> MLHAFTNQYQLSKTLRFGATLKEDEKKCKSHEELKGFVDISYENMKSSATIAESLNENELVKKCERCYSEIVKFHNAWEKIYYRTDQIAVYKDFYRQLSRKARFDAGKQNSQLITLASLCGMYQGAKLSRYITNYWKDNITRQKSFLKDFSQQLHQYTRALEKSDKAHTKPNLINFNKTFMVLANLVNEIVIPLSNGAISFPNISKLEDGEESHLIEFALNDYSQLSELIGELKDAIATNGGYTPFAKVTLNHYTAEQKPHVFKNDIDAKIRELKLIGLVETLKGKSSEQIEEYFSNLDKFSTYNDRNQSVIVRTQCFKYKPIPFLVKHQLAKYISEPNGWDEDAVAKVLDAVGAIRSPAHDYANNQEGFDLNHYPIKVAFDYAWEQLANSLYTTVTFPQEMCEKYLNSIYGCEVSKEPVFKFYADLLYIRKNLAVLEHKNNLPSNQEEFICKINNTFENIVLPYKISQFETYKKDILAWINDGHDHKKYTDAKQQLGFIRGGLKGRIKAEEVSQKDKYGKIKSYYENPYTKLTNEFKQISSTYGKTFAELRDKFKEKNEITKITHFGIIIEDKNRDRYLLASE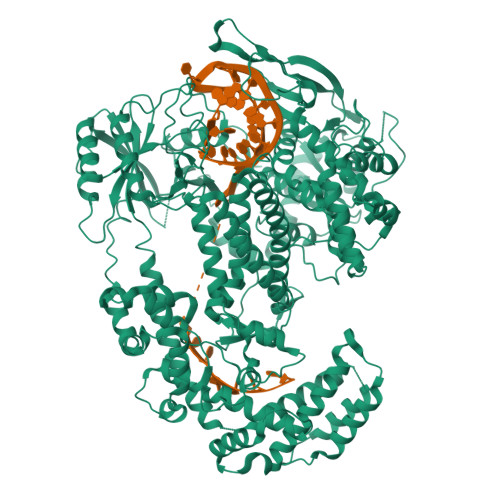LKHEQINHVSTILNKLDKSSEFITYQVKSLTSKTLIKLIKNHTTKKGAISPYADFHTSKTGFNKNEIEKNWDNYKREQVLVEYVKDCLTDSTMAKNQNWAEFGWNFEKCNSYEDIEHEIDQKSYLLQSDTISKQSIASLVEGGCLLLPIINQDITSKERKDKNQFSKDWNHIFEGSKEFRLHPEFAVSYRTPIEGYPVQKRYGRLQFVCAFNAHIVPQNGEFINLKKQIENFNDEDVQKRNVTEFNKKVNHALSDKEYVVIGIDRGLKQLATLCVLDKRGKILGDFEIYKKEFVRAEKRSESHWEHTQAETRHILDLSNLRVETTIEGKKVLVDQSLTLVKKNRDTPDEEATEENKQKIKLKQLSYIRKLQHKMQTNEQDVLDLINNEPSDEEFKKRIEGLISSFGEGQKYADLPINTMREMISDLQGVIARGNNQTEKNKIIELDAADNLKQGIVANMIGIVNYIFAKYSYKAYISLEDLSRAYGGAKSGYDGRYLPSTSQDEDVDFKEQQNQMLAGLGTYQFFEMQLLKKLQKIQSDNTVLRFVPAFRSADNYRNILRLEETKYKSKPFGVVHFIDPKFTSKKCPVCSKTNVYRDKDDILVCKECGFRSDSQLKERENNIHYIHNGDDNGAYHIALKSVENLIQMK> IVGGTASVRGEWPWQVTLHTTSPTQRHLCGGSIIGNQWILTAAHCFYGVESPKILRVYSGILNQAEIAEDTSFFGVQEIIIHDQYKMA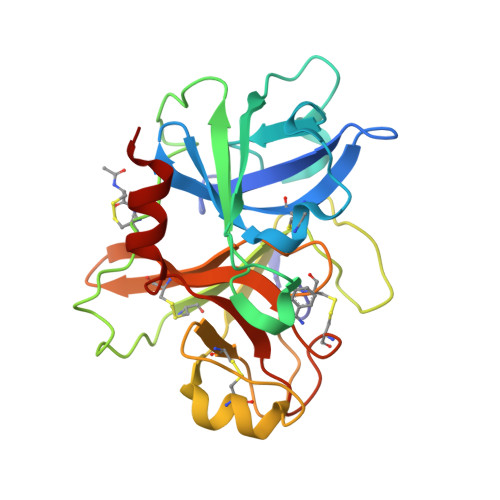ESGYDIALLKLETTVNYADSQRPICLPSKGDRNVIYTDCWVTGWGYRKLRDKIQNTLQKAKIPLVTNEECQKRYRGHKITHKMICAGYREGGKDACKGDSGGPLSCKHNEVWHLVGITSWGEGCAQRERPGVYTNVVEYVDWILEKTQAV>MRSIYLCRHGESELNLRGRIGGDSGLSARGKQYAYALANFIRSQGISSLKVWTSHMKRTIQTAEALGVPYEQWKALNEIDAGVCEEMTYEEIQEHYPEEFALRDQDKYRYRYPKGESYEDLVQRLEPVIMELERQENVLVICHQAVMRCLLAYFLDKSSDELPYLKCPLHTVLKLTPVAYGCRVESIYL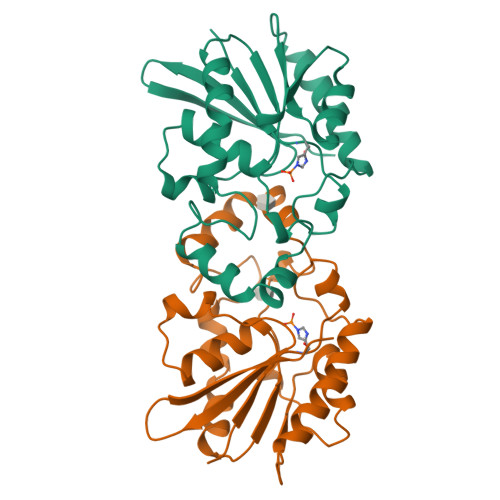NV[2x]~{N}-[4-ethanoyl-5-(4-morpholin-4-ylcarbonylphenyl)-1,3-thiazol-2-yl]piperazine-2-carboxamide | C21 H25 N5 O4 S | 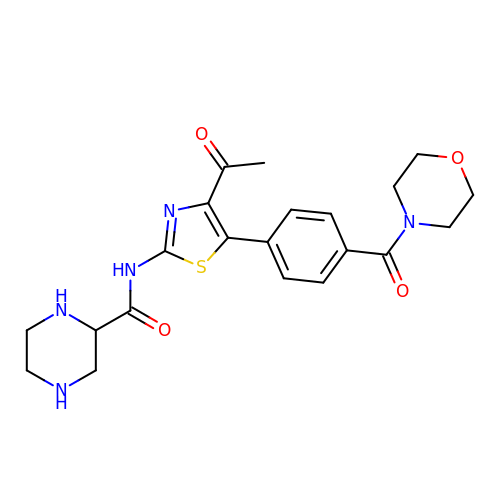ONQFETXPMZBVQB-UHFFFAOYSA-N> XREYV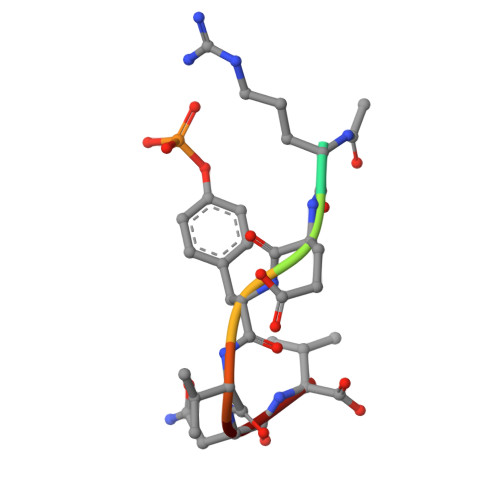NV>MSAKDERAREILRGFKLNWMNLRDAETGKILWQGTEDLSVPGVEHEARVPKKILKCKAVSRELNFSSTEQMEKFRLEQKVYFKGQCLEEWFFEFGFVIPNSTNTWQSLIEAAPESQMMPASVLTGNVIIETKFFDDDLLVSTSRVRLFYV[2x];>D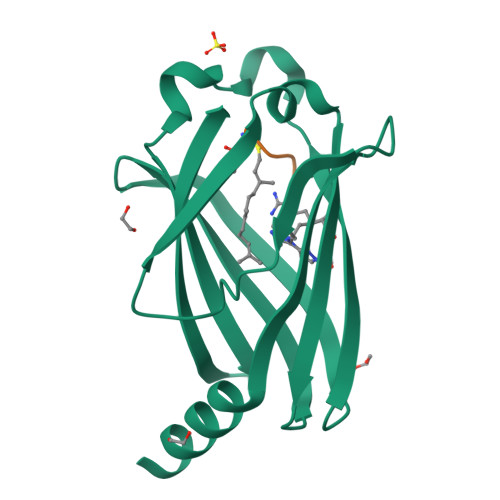GKKKKKKSKTKC[2x]> GHAADRIARLPGQPAVDFDMYSGYITVDEGAGRSLFYLLQEAPEDAQPAPLVLWLNGGPGCSSVAYGASE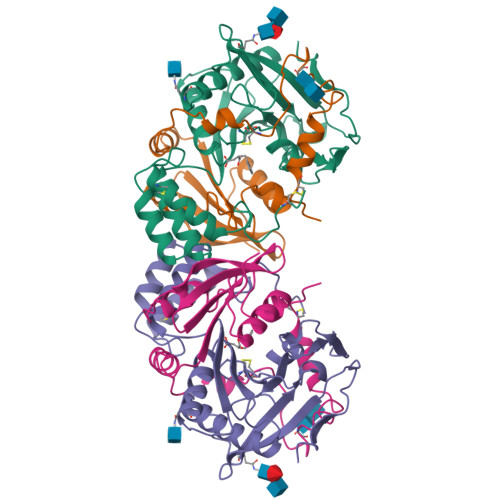ELGAFRVKPRGAGLVLNEYRWNKVANVLFLDSPAGVGFSYTNTSSDIYTSGDNRTAHDSYAFLAKWFERFPHYKYRDFYIAGESYAGHYVPELSQLVHRSKNPVINLKGFMVGNGLIDDYHDYVGTFEFWWNHGIVSDDTYRRLKEACLHDSFIHPSPACDAATDVATAEQGNIDMYSLYTPVCNI;> SYDPCTERYSTAYYNRRDVQMALHANVTGAMNYTWATCSDTINTHWHDAPRSMLPIYRELIAAGLRIWVFSGDTDAVVPLTATRYSIGALGLPTTTSWYPWYDDQEVGGWSQVYKGLTLVSVRGAGHEVPLHRPRQALVLFQYFLQGKPMPGQ> MDRASELLFYVNGRKVIEKNVDPETMLLPYLRKKLRLTGTKYGCGGGGCGACTVMISRYNPITKRIRHHPANACLIPICSLYGAAVTTVEGIGSTHTRIHPVQERIAKCHGTQCGFCTPGMVMSIYTLLRNHPEPTLDQLTDALGGNLCRCTGYRPIIDACKTFCKTSGCCQSKENGVCCLDQGINGLPEFEEGSKTSPKLFAEEEFLPLDPTQELIFPPELMIMAEKQSQRTRVFGSE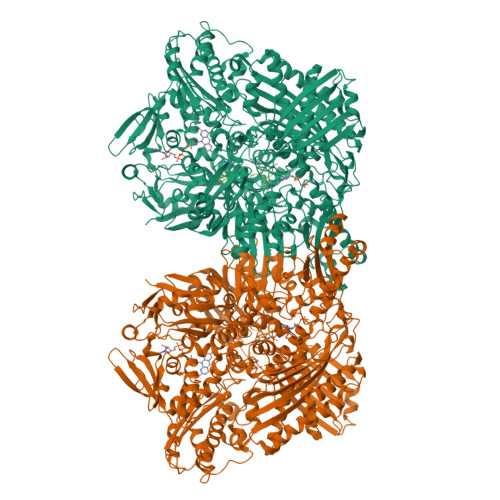RMMWFSPVTLKELLEFKFKYPQAPVIMGNTSVGPEVKFKGVFHPVIISPDRIEELSVVNHAYNGLTLGAGLSLAQVKDILADVVQKLPEEKTQMYHALLKHLGTLAGSQIRNMASLGGHIISRHPDSDLNPILAVGNCTLNLLSKEGKRQIPLNEQFLSKCPNADLKPQEILVSVNIPYSRKWEFVSAFRQAQRQENALAIVNSGMRVFFGEGDGIIRELCISYGGVGPATICAKNSCQKLIGRHWNEQMLDIACRLILNEVSLLGSAPGGKVEFKRTLIISFLFKFYLEVSQILKKMDPVHYPSLADKYESALEDLHSKHHCSTLKYQNIGPKQHPEDPIGHPIMHLSGVKHATGEAIYCDDMPLVDQELFLTFVTSSRAHAKIVSIDLSEALSMPGVVDIMTAEHLSDVNSFCFFTEAEKFLATDKVFCVGQLVCAVLADSEVQAKRAAKRVKIVYQDLEPLILTIEESIQHNSSFKPERKLEYGNVDEAFKVVDQILEGEIHMGGQEHFYMETQSMLVVPKGEDQEMDVYVSTQFPKYIQDIVASTLKLPANKVMCHVRRVGGAFGGKVLKTGIIAAVTAFAANKHGRAVRCVLERGEDMLITGGRHPYLGKYKAGFMNDGRILALDMEHYSNAGASLDESLFVIEMGLLKMDNAYKFPNLRCRGWACRTNLPSNTAFRGFGFPQAALITESCITEVAAKCGLSPEKVRIINMYKEIDQTPYKQEINAKNLIQCWRECMAMSSYSLRKVAVEKFNAENYWKKKGLAMVPLKFPVGLGSRAAGQAAALVHIYLDGSVLVTHGGIEMGQGVHTKMIQVVSRELRMPMSNVHLRGTSTETVPNANISGGSVVADLNGLAVKDACQTLLKRLEPIISKNPKGTWKDWAQTAFDESINLSAVGYFRGYESDMNWEKGEGQPFEYFVYGAACSEVEIDCLTGDHKNIRTDIVMDVGCSINPAIDIGQIEGAFIQGMGLYTIEELNYSPQGILHTRGPDQYKIPAICDMPTELHIALLPPSQNSNTLYSSKGLGELGVFLGCSVFFAIHDAVSAARQERGLHGPLTLNSPLTPEKIRMACEDKFTKMIPRDEPGSYVPWNVPI The TREX-2 complex (Transcription-Export complex 2) is conserved across eukaryotes and integrates mRNA export into the gene expression pathway and, in yeast, also mediates the location of actively-expressed genes such as GAL1 to the nuclear envelope (García-Oliver et al., 2012, Köhler and Hurt, 2007, Rodríguez-Navarro et al., 2004). The TREX-2 complex has been implicated in a spectrum of biological roles including preventing genome instability, transcription initiation, gene-gating, and mRNA export (Bhatia et al., 2014, Faza et al., 2009, Gallardo et al., 2003). We circumvented these difficulties by expressing the S. cerevisiae TREX-2 complex using a single Baculovirus harboring the cDNA coding sequences of one copy of Sac3, Thp1, Sem1, Cdc31, and Sus1. Complementary structural analysis of this material has demonstrated that in contrast to the previously characterized TREX-2 complex from C. thermophilum that the CID-subcomplex is likely not to have a defined spatial arrangement with respect to the M-subcomplex and that the TPR-like repeat region of the Sac3 chain extends further towards the N-terminus than had been previously thought.

Crystals with P212121 symmetry with a = 78.2 Å, b = 84.1 Å, c = 165.5 Å that diffracted to 4.9 Å resolution using synchrotron radiation were obtained of the TREX-2 complex. However, the volume of the asymmetric unit (1,087,701 Å3) would only have accommodated the entire complex if the solvent content was of the order of 12% and so it was likely that they instead contained a proteolytic fragment of the complex. Consistent with this hypothesis, limited proteolysis experiments showed that in the TREX-2 complex Sac3 was cleaved by both trypsin and chymotrypsin to yield a stable fragment at about ∼60 kDa. The TPR-like repeat helices and the winged helix domains of both Sac3 and Thp1 were clear, although in places the density corresponding to some of the loops was less clear. Unfortunately it was not possible to identify unequivocally the residues linking these helices and so, because the density due to the side chains in these cylinders was not sufficiently clear to enable individual residues to be assigned unequivocally and so they were modeled as polyAla. No other difference density was observed that could correspond to the CID domain of the complex (containing Sac3 residues 727–805, together with two Sus1 chains and a Cdc31 chain), consistent with the crystals containing only the N-terminal half of Sac3 (up to about residue 555) together with Thp1 and Sem1. Although the material used in crystallization trials contained Sac3 residues 1–805, it was likely that, as is commonly observed, the CID-subcomplex and possibly also residues at the Sac3 N-terminus had been removed during the 2 weeks needed for the crystals to grow. Consistent with the possibility, micro-seeding attempts using these crystals in crystallization trials using freshly-prepared complex were unsuccessful.

> MNTSFGSVVPSTNFNFFKGHGNNDNTSANSTVNNSNFFLNSNETKPSKNVFMVHSTSQKKSQQPLQNLSHSPSYTENKPDKKKKYMINDAKTIQLVGPLISSPDNLGFQKRSHKARELPRFLINQEPQLEKRAFVQDPWDKANQEKMISLEESIDDLNELYETLKKMRNTERSIMEEKGLVDKADSAKDLYDAIVFQGTCLDMCPTFERSRRNVEYTVYSYEKNQPNDKKASRTKALKVFARPAAAAAPPLPSDVRPPHILVKTLDYIVDNLLTTLPESEGFLWDRMRSIRQDFTYQNYSGPEAVDCNERIVRIHLLILHIMVKSNVEFSLQQELEQLHKSLITLSEIYDDVRSSGGTCPNEAEFRAYALLSKIRDPQYDENIQRLPKHIFQDKLVQMALCFRRVISNSAYTERGFVKTENCLNFYARFFQLMQSPSLPLLMGFFLQMHLTDIRFYALRALSHTLNKKHKPIPFIYLENMLLFNNRQEIIEFCNYYSIEIINGDAADLKTLQHYSHKLSETQPLKKTYLTCLERRLQKTTYKGLINGGEDNLASSVYVKDPKKDRIPSIADQSFLMENFQNNYNEKLNQNSSVKPQINTSPKRVATRPNHFPFSQESKQLPQISQSHTLSTNPLLTPQVHGDLSEQKQQQIKTVTDGGSPFVFDQSAQNSTVEASKAHMISTTSNGAYDEKLSSEQEEMRKKEEQRIEEEKTQLKKKQENADKQVITEQIANDLVKEVVNSSVISIVKREFSEANYRKDFIDTMTRELYDAFLHERLYLIYMDSRAELKRNSTLKKKFFEKWQASYSQAKKNRILEEKKREEIKLVSHQLGVPGFKKSTCLFRTPYKGNVNSSFMLSSSDKNLIFSPVNDEFNKFATHLTKISKLWRPLEMQSIYYDNLTKKFPSNSLTPANLFIYAKDWTSLSNRWILSKFNLQTAQDSKKFSNNIISSRIICIDDEYEPSDFSDLQLLIFNTGVTNPDIFDLEMKLKDDGEELIKLITGISLNTNICFSLLIIYWESAENTLSESTIKHLLKLNRISKNYSSVIERIDLMNLTEESPHKCLEDKLSEISHSYVYKLTERGKYDKTLRQKRSLAGIHSRSTQLQTTKDIDQKMKKMLEKEKNKYQQQIGERNTYAHLESHIDASPRSKKRKLPILLSTSHSSQFKTPLASRLNTSGSSTSPPLPSHLAMKFRKNSRVTSLHTVLPVSTPSHSNNIPAASFSGNNTTDIQSQQLIENQKSTSVYLNNVSERILGNQEICQTPINPVTPVLDGADQGKEDIPDSILELKILIDSVKKKVNND;> MDMANQLLDELAHGNFSHLTLNLSQNGREIAILQKQLTGFDDKQLETFVEQHPAMPNDTRFKIMCTSFLNYARDVDPWSAWSSSDLIFEFYQCLINCLINDNAPHIEMLIPVATRETEFIINLAGKLDSFHLQLHTRSHQFLSHISSILSRLFNSIKPPRGNASSTNIPGKQRILLYLVNKLNNIYFRIESPQLCSNIFKNFQPKSMLAHFNEYQLDQQIEYRYLLGRYYLLNSQVHNAFVQFNEAFQSLLNLPLTNQAITRNGTRILNYMIPTGLILGKMVKWGPLRPFLSQETIDNWSVLYKHVRYGNIQGVSLWLRQNERHLCARQLLIVLLEKLPMVTYRNLIKTVIKSWTTEWGQNKLPYSLIERVLQLSIGPTFEDPGAQEITIYNGIHSPKNVENVLVTLINLGLLRANCFPQLQLCVVKKTTMIQEIVPPVNERITKMFPAHSHVLW;> MSTDVAAAQAQSKIDLTKKKNEEINKKSLEEDDEFEDFPIDTWANGETIKSNAVTQTNIWEENWDDVEVDDDFTNELKAELDRYKRENQ> MITILDYLFLLDLNDDLTRKAVFEQVIIFIFIYCTMNFLAWSTVVELIWPTHF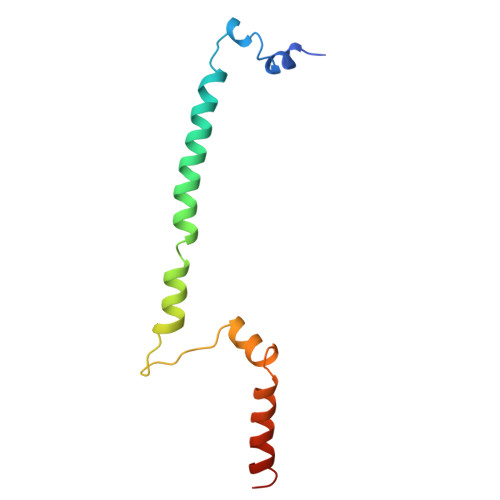FNRRHSSSQEFIRFRTYTEVLLKISAYNDFFYVLNNYYYNQKLILKN> MGPSLDFALSLLRRNIRQVQTDQGHFTMLGVRDRLAILPRHSQPGKTIWVEHKLINVLDAVELVDEQGVNLELTLVTLDTNEKFRDVTKFIPETITGASDATLIINTEHMPSMFVPVGDVVQYGFLNLSGKPTHRTMMYNFPTKAGQAGGVVTSVGKII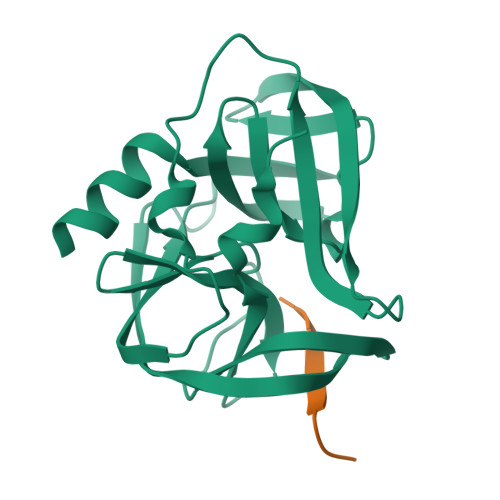GIHIGGNGRQGFCAGLKRGYFASEQHHHHHH;> FAGLRQAVTQ>[6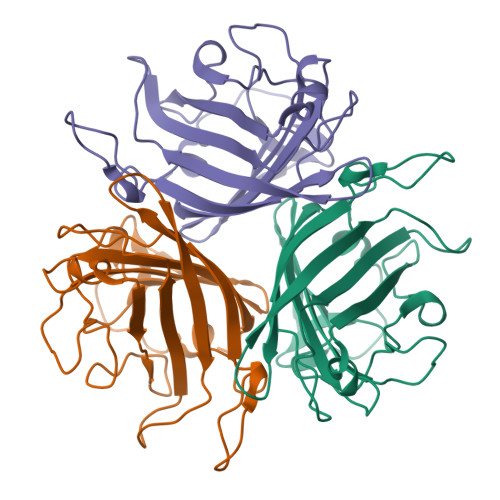x]GSHMASMTGGQQMGRGSDSSNAITIENNTLWTGAKPSANCVIKEGEDSPDCKLTLVLVKNGGLINGYITLMGASEYTNTLFKNNQVTIDVNLAFDNTGQIITYLSSLKSNLNFKDNQNMATGTITSAKGFMPSTTAYPFITYATETLNEDYIYGECYYKSTNGTLFPLKVTVTLNRRMLASGMAYAMNFSWSLNAEEAPETTEVTLITSPFFFSYIREDD>[3x]QKPNIILIVADDLGYADVGFNGSKDIITPNIDDLAKSGTSFSDAYVAHPFSGPSRAALMTGRYPHKIGSQFNLPTRGSN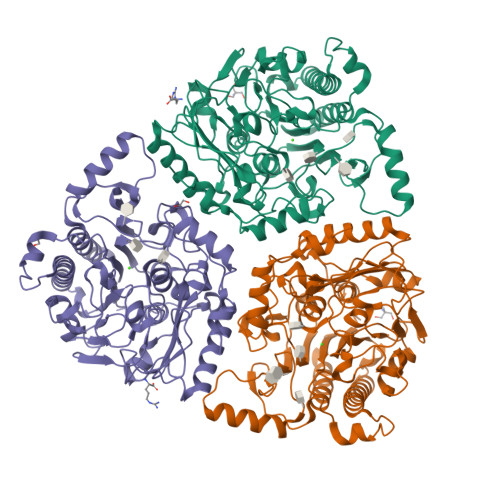VGVPTDAKFISKLLNENNYFTGALGKWHMGDTPQHHPNKRGFDEYYGFLGGGHNYFPDQYQPQYKKQKAQGLKNIFEYITPLEHNGKEVKETQYITDALSREAVNFVDKAVNKKHPFFLYLAYNAPHTPLQAKDEDMAMFPNIKNKDRKTYAGMVYAVDRGVGKLVEALKKNNQYDNTLIVFMSDNGGKLSKGANNFPLKAGKGSTQEGGFRVPMLFHWPKHVPAGKRFSHPVSALDLYPTFAALAGAKVEENQHLDGTNMWPAFIKNENPHKDEPIYALRHRKGYSDAAIRMNQWKALKVNQQPWQLFNIENDISEKHDVSKSNKALLTDMVREMEKWSWDNQQPSWFHETTEGVNWRLDAMPRFDKTFKTT> MQQLNENKIIKLLRDNIPKLQLIYLFGSYSQGTQHRNSDIDIAVLAADTLDNIARWELAQKLASALDSDVDLVDLRSASTVLCQQVVTQGKQLWGTQQDDELFAVKTISMY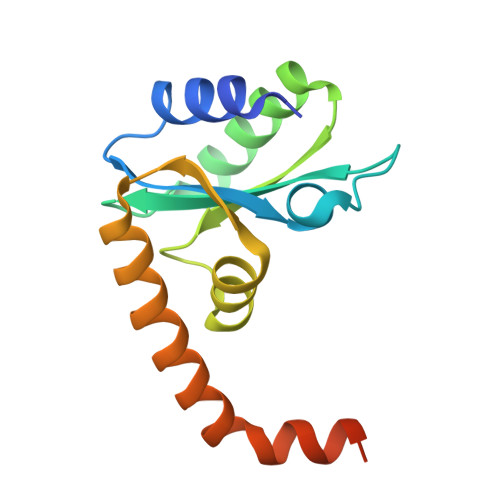QHLQAERQAIIDDVMANTAAKAHRGESL>APADNAADARPVDVSVSIFINKIYGVNTLEQTYKVDGYIVAQWTGKPRKTPGDKPLIVENTQIERWINNGLWVPALEFINVVGSPDTGNKRLMLFPDGRVIYNARFLGSFSNDMDFRLFPFDRQQFVLELEPFSYNNQQLRFSDIQVYTENIDNEEIDEWWIRKASTHISDIRYDHLSSVQPNQNEFSRITVRIDAVRNPSYYLWSFILPLGLIIAASWSVFWLESFSERLQTSFTLMLTVVAYAAYTSNILPRLPYTTVIDQMIIAGYGSIFAAILLIIFAHHRQANGVEDDLLIQRCRLAFPLGFLAIGCVLVIRGITL[10x]

The pentameric ligand-gated ion channels (pLGICs) constitute a large family of ionotropic neurotransmitter receptors that are ubiquitously expressed in the animal kingdom. The proteins act as gated ion channels that are closed in their resting state and that open a selective ion conduction pore upon the binding of a ligand to a site located on an extracellular domain. ELIC is activated by a set of primary amines that include alkylamines, aminothiols, aminoalcohols, bromoamines, diamines, and the neurotransmitter GABA. ELIC is a cation selective channel that is essentially impermeable for anions.

In cation selective pLGICs, three layers of hydrophobic side-chains provide an overall apolar character to the extracellular half of the pore region while the following two layers of polar residues and a layer of negatively charged residues render the intracellular half hydrophilic. In a recent study, it was suggested that interactions between aromatic residues (i.e., Phe246) of the outer hydrophobic layer would stabilize the closed conformation of ELIC. To investigate the role of this aromatic group for channel opening, we have mutated it to alanine and studied the mutant by X-ray crystallography and electrophysiology. The structure of the mutant F246A was determined at 3.3 Å resolution and shows a conformation that is, apart from the side chain truncation, virtually identical to WT. In electrophysiological recordings we found that the EC50 of cysteamine activation of F246A was shifted towards higher concentrations. This shift is due to a mutation of a residue located remote from the ligand binding site and thus likely reflects a decreased efficacy of the channel. Our results thus do not provide any evidence that the ring of phenylalanine residues, which is unique to ELIC, would stabilize the pore in an unusual non-conducting conformation. A previous hypothesis that the observed conformation would be induced by strong interactions of aromatic phenylalanine residues at the extracellular pore entry, however, could not be substantiated since the mutation to alanine did not change the overall structure and instead stabilized the closed state of the channel as indicated by a decrease in the potency of the agonist. This observation is unexpected, as hydrophobic interactions generally play an important role in the stabilization of protein structures. While the bulky Phe246 and Leu239 at the extracellular half of the pore of ELIC would result in a smaller pore diameter, the constricting intracellular diameter, which might be the main determinant for the conductance, could be larger.> DVPVNLYRPNAPFIGKVISNEPLVKEGGIGIVQHIKFDLTGGNLKYIEGQSIGIIPPGVDKNGKPEELRLYSIASTRHGDDVDDKTISLCVRQLEYKHPESGETVYGVCSTYLTHIEPGSEVKITGPVGKEMLLPDDPEANVIMLATGTGIAPMRTYLWRMFKDAERAANPEYQFKGFSWLVFGVPTTPNILYKEELEEIQQKYPDNFRLTYAISREQKNPQGGRMYIQDRVAEHAD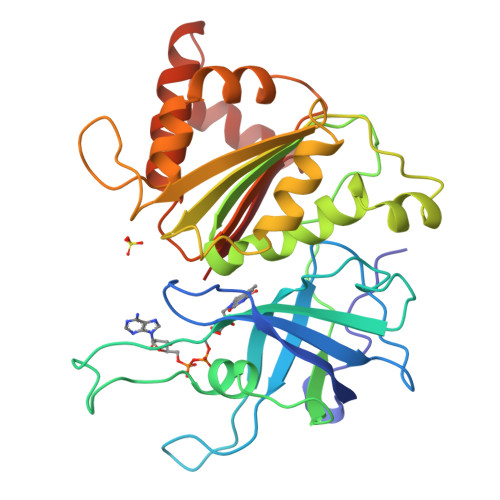QLWQLIKNQKTHTYICGLRGMEEGIDAALSAAAAKEGVTWSDYQKDLKKAGRWHVETY> KAGPTLEELLGQCTAENRHHEYLCDSQGKE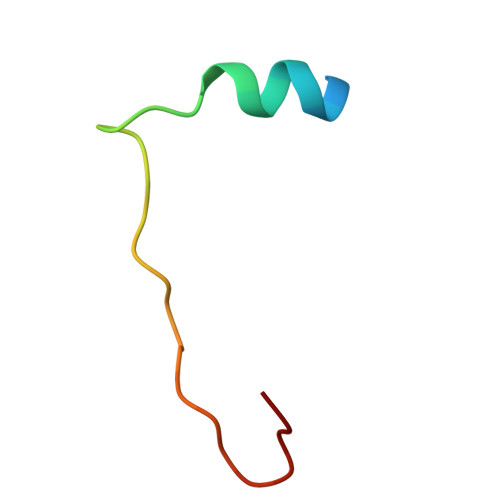ML>SNAVRGFLIVGNKAFTQPFSLNDLPGAGRMDVLCRCTSQALFISHGIRRDVEVYLLLLGPPSPPKSILIKGDEVRRMSPDERNVAGHIKKALAVECGKSWKKVHSGVYVSRKGLEELIEELSEKYSIIYLKEDGVDISNAQLPPNPLFVIGDHE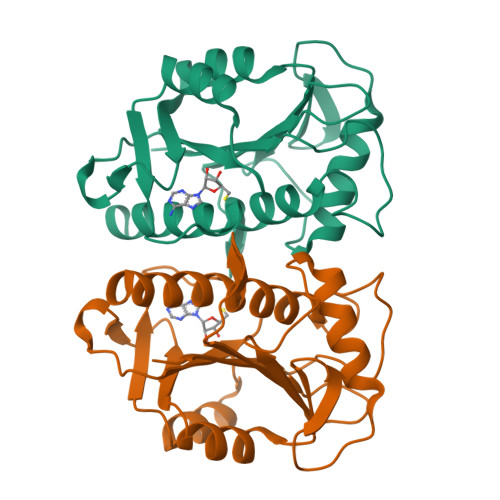GLTEEQEKVVERYAALKLSLSPLSLLAEQCVVIAHHHLDRLQF[2x]> MFKAQATFSRYSAAVSLLLLFSGAAQAAPQSITTLPLQPDGENRWRLPAGEYQGQFTIEQPMQLRCEPGAVIQSQGQGSSLLISAPDVLVEGCTLYEWGSDLTAMDSAVFILPAAERAQISNNRMRGPGFGVFVDGTRDVQVIGNEIDGDAGVRSQDRGNGIHLFAVSGARVLHNHVRNARDGIYIDTSNGNHLEGNVIEDVRYGVHYMFANENSLIDNVTRRTRTGYALMQSRKLTVTGNRSEQDQNYGILMNYITYSTITGNFVSDVQRGDTGGDSMISGGEGKALFIYNSLFNTIENNHFEKSSLG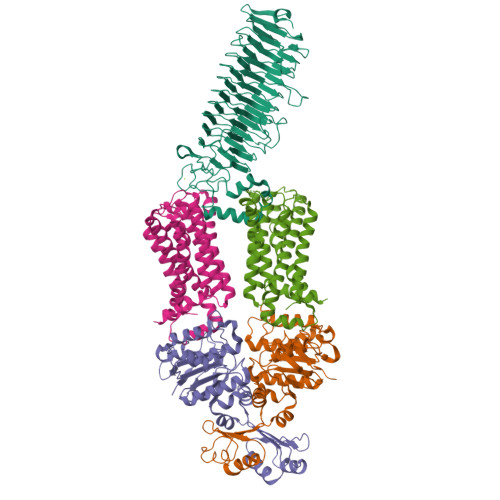IHLTAGSEDNRISGNAFVGNQQQVKYVASRTQEWSVDGRGNYWSDYLGWDRNNDGLGDIAYEPNDNVDRLLWLYPQVRLLMNSPSIEVLRWVQRAFPVIKSPGVQDSHPLMKLPTEKLLTEKQEPTS;>MNAVEIQGVSQRYGSMTVLHDLNLNLGEGEVLGLFGHNGAGKTTSMKLILGLLSPSEGQVKVLGRAPNDPQVRRQLGYLPENVTFYPQLSGRETLRHFARLKGAALTQVDELLEQVGLAHAADRRVKTYSKGMRQRLGLAQALLGEPRLLLLDEPTVGLDPIATQDLYLLIDRLRQRGTSIILCSHVLPGVEAHINRAAILAKGCLQAVGSLSQLRAEAGLPVRIRASGISERDSWLQRWTDAGHSARGLSESSIEVVAVNGHKLVLLRQLLGEGEPEDIEIHQPSLEDLYRYYMERAGDVRAQEGRL[2x];>MNQVWNIARKELSDGLRNRWLLAISLLFAVLAVGIAWLGAAASGQLGFTSIPATIASLASLATFLMPLIALLLAYDAIVGEDEGGTLMLLLTYPLGRGQILLGKFVGHGLILALAVLIGFGCAALAIALLVEGVELGMLFWAFGRFMISSTLLGWVFLAFAYVLSGKVNEKSSAAGLALGVWFLFVLVFDLVLLALLVLSEGKFNPELLPWLLLLNPTDIYRLINLSGFEGSGSAMGVLSLGADLPVPAAVLWLCLLAWIGVSLLLAYAIFRRRLT[2x]> GVMTDVHRRFLQLLMTHGVLEEWDVKRLQTHCYKVHDRNATVDKLEDFINNINSVLESLYIEIKRGVTEDDGRPIYALVNLATTSISKMATDFAENELDLFRKALELIIDSETGFASSTNILNLVDQLKGKKMRKKEAEQVLQKFVQNKWLIEKEGEFTLHGRAILEMEQYIRETYPDAVKICNICHSLLIQGQSCETCGIRMHLPCVAKYFQSNAEPRCPHCNDYWPHEIPKVFDPE;> GPRSQKQLELKVSELVQFLLIKDQKKIPIKRADILKHVIGDYKDIFPDLFKRAAERLQYVFGYKLVELEPKSNTYILINTLEPVEEDAEMRGDQGTPTTGLLMIVLGLIFMKGNTLKETEAWDFLRRLGVYPTKKHLIFGDPKKLITED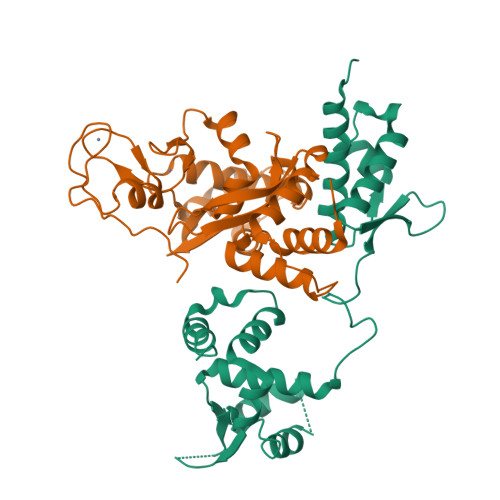FVRQRYLEYRRIPHTDPVDYEFQWGPRTNLELSKMKVLKFVAKVHNQDPKDWPAQYCEALADEENRAR> MVCKVCGQKAQVEMRSRGLALCREHYLDWFVKETERAIRRHRMLLPGERVLVAVSGGKDSLALWDVLSRLGYQAVGLHIELGIGEYSKRSLEVTQAFARERGLELLVVDLKEAYGFGVPELARLSGRVACSACGLSKRYIINQVAVEEGFRVVATGHNLDDEAAVLFGNLLNPQEETLSRQGPVLPEKPGLAARVKPFYRFSEREVLSYTLLRGIRYLHEECPNAKG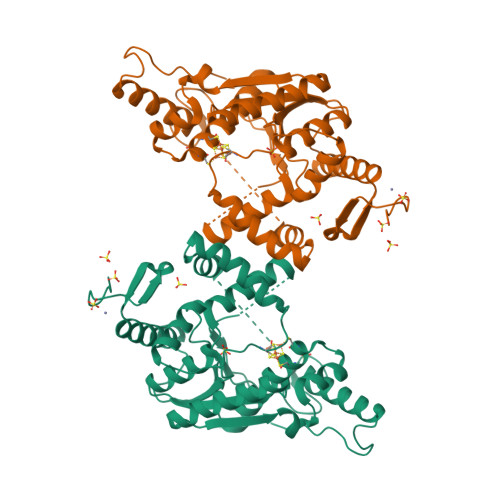AKSLLYKEALNLVERSMPGAKLRFLDGFLEKIRPRLDVGEEVALRECERCGYPTTGAVCAFCRMWDAVYRRAKKRKLLPEEVSFRPRVKPLRAGVEHHHHHH2-(3-METHYLPHENYL)-1H-INDOLE-5-CARBOXIMIDAMIDE 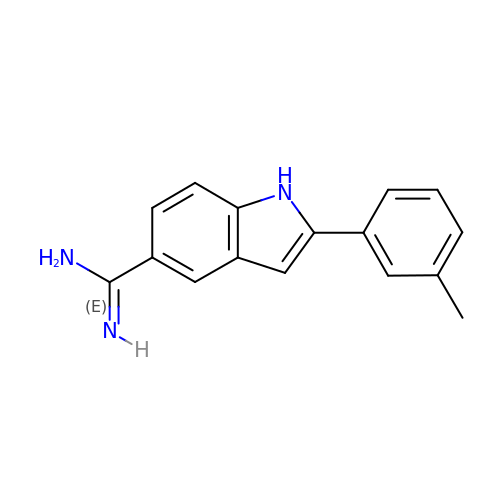| C16 H15 N3 | KJUSXMYSVXZFDJ-UHFFFAOYSA-N> AMVSMKEFIGRWKLVHSENFEEYLKEIGVGLLIRKAASLTSPTLEIKLDGDTWHFNQYSTFKNNKLAF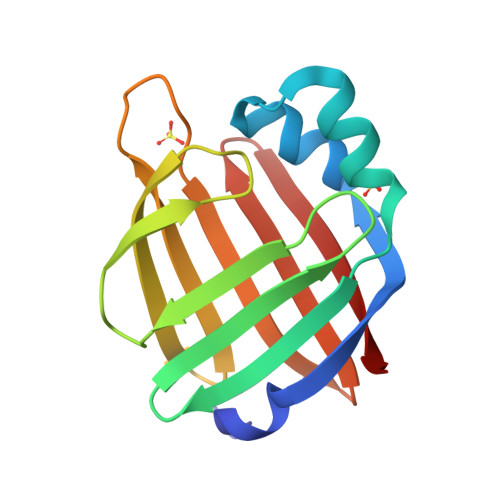KIREKFVEIAPDERSYNTLVTFENGKFISHQDKIKENHHSSVFTTWLENGKLLQTYQSGSVICRREFVKE>SNAMPMTIKRATWNNGPDLAFDINNKANAAIEKYGREAVINAALGTLLDDKGKIIALPSVYDRLDEMDRSHIASYAPIEGEKDYRKIVIDTLFGPYKPEGYISAIATPGGTGAIRSAIFSYLDEGDPLICHDYYWAPYRKICEEFGRNFKTFEFFTDDFAFNIDVYKEAIDEGIRDSDRIASLINSPGNNPTGYSLSDEEWDEVITFLKEKAEDKDKKITLIVDVAYLEFAGDGDQQRKFFEKFSNLPRNLFVVVAFSMSKSHTAYGLRSGAAVGI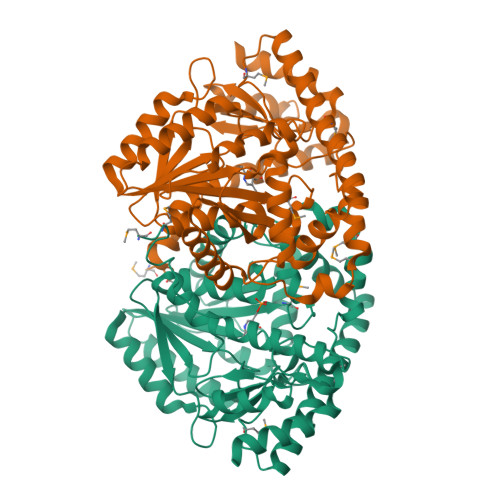SSSKEIIEEFEASLAHSARCNWSNGTHAAQNILIELERAENKKIYEQELVDLRNMLKSRADVFVTAAKENKLTMIPYFGGFFTFIPTDKAFDIVKDLEKENIFTIPSAKGIRVAICGVGEEKIPKLVQRLAFYTNKK[4x]>MKSEKEKMLAGHLYNPADLELVKERERARRLVRLYNETLETEYDKRTGLLKELFGSTGERLFIEPNFRCDYGYNIHVGENFFMNFDGVILDVCEVRIGDHCFIGPGVHIYTATHPLDPHERNSGLEYGKPVVIGHNVWIGGRAVINPGVTIGDNAVIASGAVVTKDVPANAVVGGNP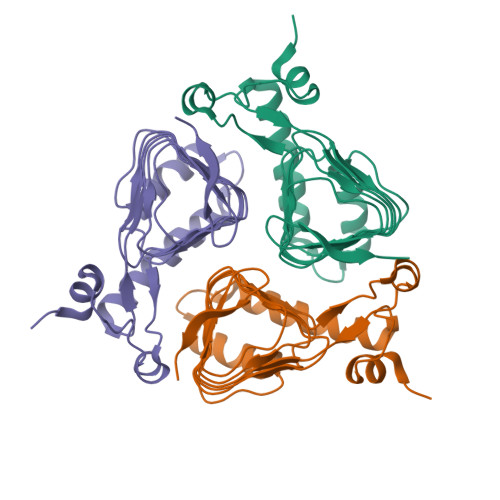AKVIKWLK[3x]>[4x]MGSDKIHHHHHHENLYFQGMGTDKFNNIKIDKYENLINVLKTGDIFLCSGNYLVSKLIKKVSESM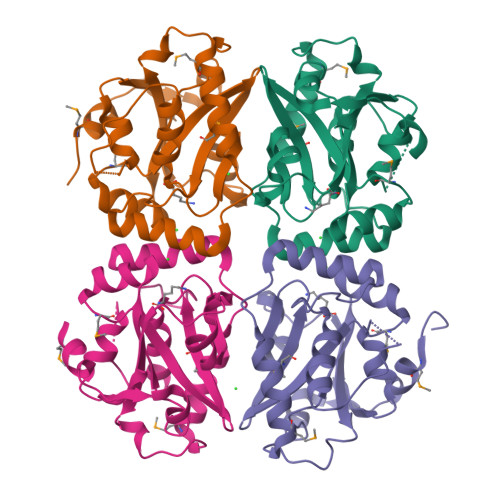FSHTGIIVKWGEHTLIMESVEDDGVRIVPLEHYIKNYENSNNRYNGSLFIARHELLQNVNDDSEMIRNLIKVGFSLLNSGYDKNEIAQIVARIGLGIGRHEDNNEYICSEFVNECFKKIGVEFLTDSEGFIFPEHIAADHHVLPIAQIE>VSQIYQVSTMTSLLDGVYDGDFELSEIPKYGDFGIGTFNKLDGELIGFDGEFYRLRSDGTATPVQNGDRSPFCSFTFFTPDMTHKIDAKMTREDFEKEINSMLPSRNLFYAIRIDGLFKKVQTRTVELQEKPYVPMVEAVKTQPIFNFDNVRGTIVGFLTPAYANGIAVSGYHLHFIDEGRNSGGHVFDYVLEDCTVTISQKMNMNLRLPNTADFFNANLDNPDFAKDIETT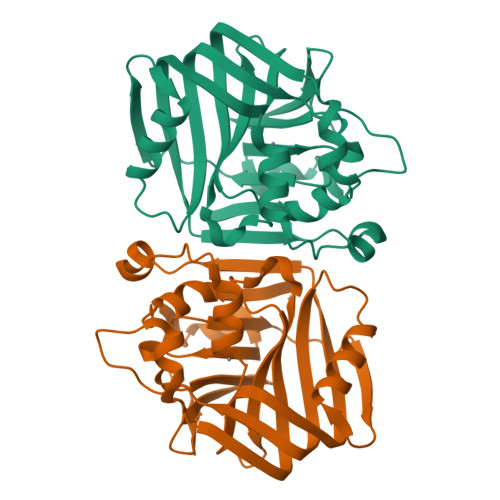EGS[2x]(2S)-2-cyclohexyl-2-{5,6-difluoro-2-[(R)-methoxy(phenyl)methyl]-1H-benzimidazol-1-yl}-N-(trans-4-hydroxycyclohexyl)acetamide | C29 H35 F2 N3 O3 | 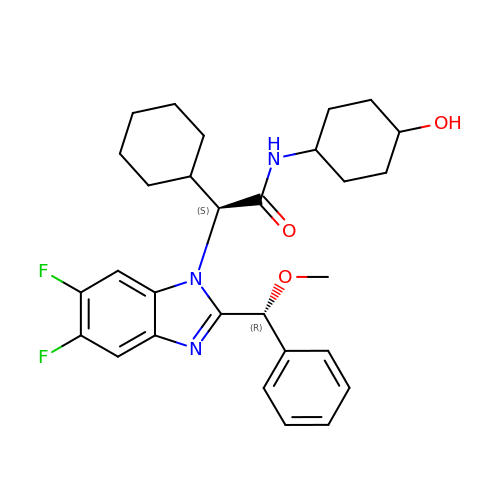JJRPVOCGGUAZIT-LKSLQULUSA-N> MAPEYWCSIAYFEMDVQVGETFKVPSSCPIVTVDGYVDPSGGDRFCLGQLSNVHRTEAIERARLHIGKGVQLECKGEGDVWVRCLSDHAVFVQSYYLDREAGRAPGDAVHKIYPSAYIKVFDLRQCHRQMQQQAATAQAAAAAQAAAVAGNIPGPGSVGGIAPAISLSAAAGIGVDDLRRLCILRMSFVKGWGPDYPRQSIKETPCWIEIHLHRALQLLDEVLHTMPIADPQP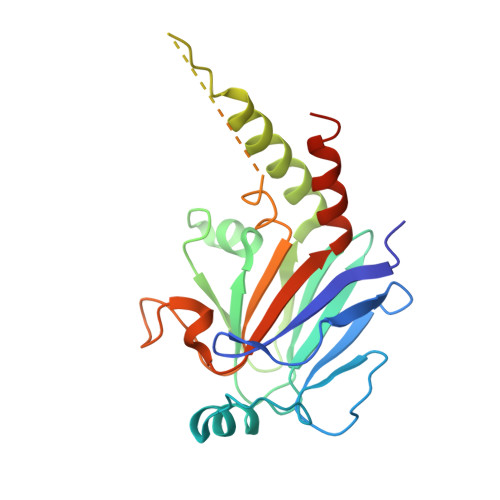LD> MHHHHHHHHHHSSGLVPRGSHRILNLVKYDLYSIFKSPLTYLAILVVSSLIATQSILMANSMDNPKHIIVYGSVFAAAKWLLLIIGLMFVVKTITRDFSQGTIQLYMSKVKTRVGYII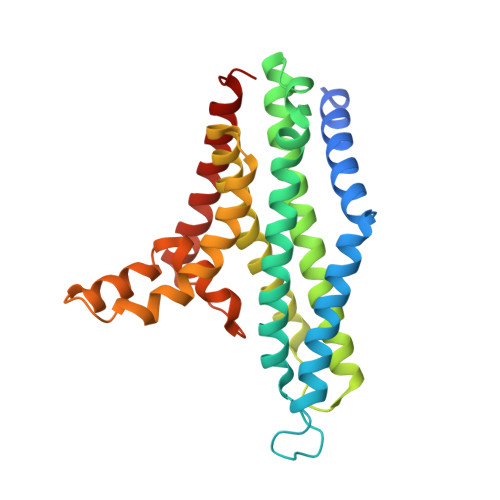SKTISIILISILFALIHYVILIVVQASSNGKNLAFSKYVDNLWFFLIFLLFFGLFLFLITLASQKTAMIFSLGVFLVLIVPFIKPFITFIPRYGEKVLDAFDYIPFAYLTDKMISSNFDFSNWQWVISLGSIVIFFILNILYVAKKDI>MATAHFVLIHTICHGAWIWYKLKPLLEAAGHKVTALDLAASGIDPRQIEQINTFDEYSEPLLTFMESLPQGEKVILVGESCGGLNIALAADKYPEKISAAVFHNALMPDTEHSPSYVVDKFMEVFPDWKDTEFSTYTSNNETITGMKLGFKLMRENLYTNCPIEDYELAKMLTRKGSFFQNDLAQRPKFTEEGYGSIKRVYVWTDEDKIFPPEFQLWQIENYKPDKVYRVQGGDHKLQLSKTNELAEILQEVADTYADLLAVAGLEHHHHHH[4x]

A reconstructed ancestral hydroxynitrile lyase, HNL1, from the α/β-hydrolase-fold superfamily is the focus of this paper. Most enzymes in the α/β-hydrolase-fold superfamily are esterases, which catalyze the hydrolysis of esters, but this superfamily also includes lyases, which catalyze the cleavage of hydroxynitriles and the corresponding reverse addition reaction. HNL1 primarily catalyzes the cleavage of hydroxynitriles, but can also catalyze promiscuous ester hydrolysis.

The model contained six glycerol molecules, including one in each active site, and 192 water molecules. Crystallographic refinement resulted in a model to 1.96-Å resolution with an Rwork/Rfree of 9.0/11.6%, and other statistics listed in Table 3. The asymmetric unit contains a dimer of dimers. Therefore, the native arrangement of HNL1 is as the dimer like the modern hydroxynitrile lyases discussed here. The catalytic domain consists of residues 1–107 and 180–265 and contains the catalytic triad (Ser 80, His 235, and Asp 207) as well as the catalytic Lys 236. The overall structure of HNL1 is similar to that of modern hydroxynitrile lyases HbHNL, MeHNL, and BmHNL. The larger phenylalanines in HNL1 push the side chain of Trp128 out of the active site by 1.3 Å as compared to HbHNL (1 Å relative to MeHNL), thereby creating a larger substrate-binding region in HNL1. The active site volume of HNL1 (143 Å3) is larger than the active site volumes of HbHNL (94–119 Å3) and esterase SABP2 (123 Å3). In addition to a larger substrate-binding region in HNL1 as compared to HbHNL, this substrate-binding region is more dynamic in HNL1.>[3x]MRIMAYQPVRRVKSGIPGFDELIEGGFPEGTTVLLTGGTGTGKTTFAAQFIYKGAEEYGEPGVFVTLEERARDLRREMASFGWDFEKYEKEGKIAIVDGVSSVVGLPSEEKFVLEDRFNVDNFLRYIYRVVKAINAKRLVIDSIPSIALRLEEERKIREVLLKLNTILLEMGVTTILTTEAPDPQHGKLSRYGIEEFIARGVIVLDLQEKNIELKRYVLI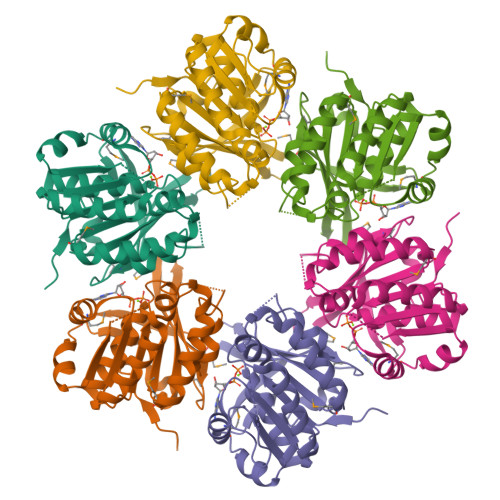RKMRETRHSMKKYPFEIGPNGIVVYPSGEIY> MPVLNLNDPQAVERYEEFMRQSPYGQVTQDLGWAKVKNNWEPVDVYLEDDQGAIIAAMSMLLGDTPTDKKFAYASKGPVMDVTDVDLLDRLVDEAVKALDGRAYVLRFDPEVAYSDEFNTTLQDHGYVTRNRNVADAGMHATIQPRLNMVLDLTKFPDAKTTLDLY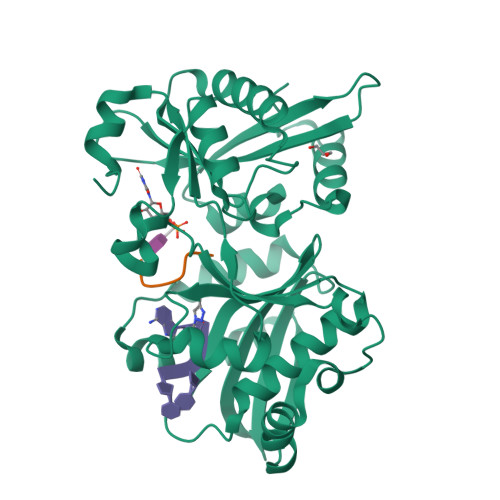PSKTKSKIKRPFRDGVEVHSGNSATELDEFFKTYTTMAERHGITHRPIEYFQRMQAAFDADTMRIFVAEREGKLLSTGIALKYGRKIWYMYAGSMDGNTYYAPYAVQSEMIQWALDTNTDLYDLGGIESESTDDSLYVFKHVFVKDAPREYIGEIDKVLDPEVYAELVKDGHHHHHH;> AECAA>[2x]GPSFWLGNETLKVPLALFALNRQRLCERLRKNPAVQAGSIVVLQGGEETQRYCTDTGVLFRQESFFHWAFGVTEPGCYGVIDVDTGKSTLFVPRLPASHATWMGKIHSKEHFKEKY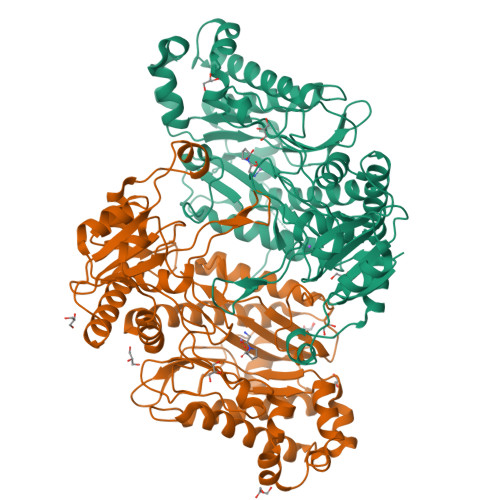AVDDVQYVDEIASVLTSQKPSVLLTLRGVNTDSGSVCREASFDGISKFEVNNTILHPEIVECRVFKTDMELEVLRYTNKISSEAHREVMKAVKVGMKEYELESLFEHYCYSRGGMRHSSYTCICGSGENSAVLHYGHAGAPNDRTIQNGDMCLFDMGGEYYCFASDITCSFPANGKFTADQKAVYEAVLRSSRAVMGAMKPGVWWPDMHRLADRIHLEELAHMGILSGSVDAMVQAHLGAVFMPHGLGHFLGIDVHDVGGYPEGVERIDEPGLRSLRTARHLQPGMVLTVKPGIYFIDHLLDEALADPARASFLNREVLQRFRGFGGVRIEEDVVVTDSGIELLTCVPRTVEEIEACMAGCDKAFTPF5-methoxy-N-(methylsulfonyl)-1H-indole-2-carboxamide | C11 H12 N2 O4 S | 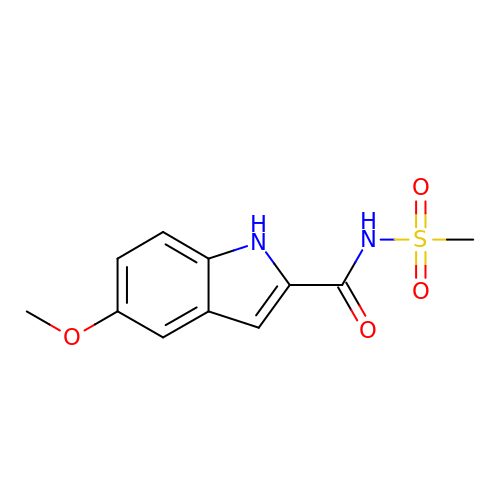DXGOZIMONBKDBI-UHFFFAOYSA-N>[2x]GSHMQEESRCQRCISELKDIRLQLEACETRTVHRLRLPLDKEPARECAQRIAEQQKAQAEVEGLGKGVARLSAEAEKVLALPEPSPAAPTLRSELELTLGKLEQVRSLSAIYLEKLKTISLVIRGTQGAEEVLRAHEEQLKEAQAVPATLPELEATKASLKKLRAQAEAQQPTFDALRDELRGAQEVGERLQQRHGERDVEVERWRERV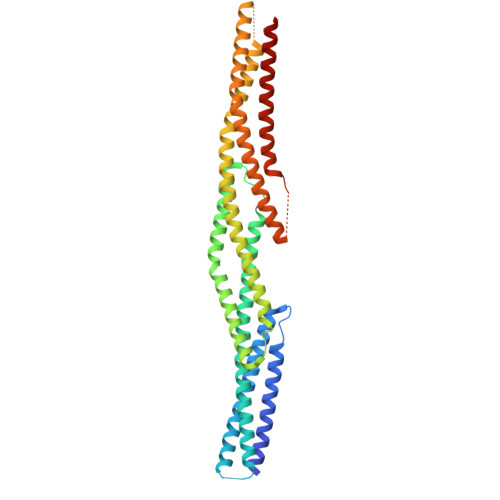AQLLERWQAVLAQTDVRQRELEQLGRQLRYYRESADPLGAWLQDARRRQEQIQAMPLADSQAVREQLRQEQALLEEIERHGEKVEECQRFAKQYINAIKDYELQLVTYKAQLEPVASPAKKPKVQSGSESVIQEYVDLRTHYSELTTLTSQYIKFISETLRRME> HSELLVN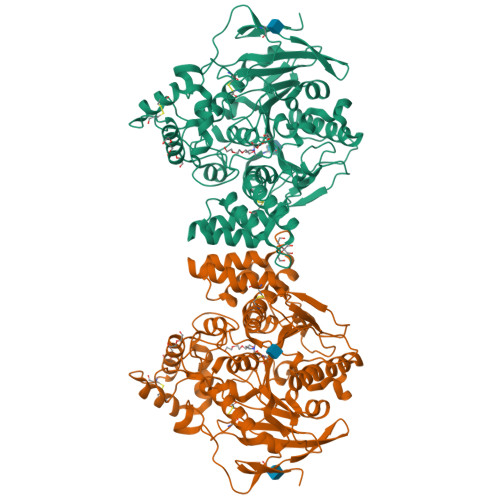TKSGKVMGTRVPVLSSHISAFLGIPFAEPPVGNMRFRRPEPKKPWSGVWNASTYPNNCQQYVDEQFPGFSGSEMWNPNREMSEDCLYLNIWVPSPRPKSTTVMVWIYGGGFYSGSSTLDVYNGKYLAYTEEVVLVSLSYRVGAFGFLALHGSQEAPGNVGLLDQRMALQWVHDNIQFFGGDPKTVTIFGESAGGASVGMHILSPGSRDLFRRAILQSGSPNCPWASVSVAEGRRRAVELGRNLNCNLNSDEELIHCLREKKPQELIDVEWNVLPFDSIFRFSFVPVIDGEFFPTSLESMLNSGNFKKTQILLGVNKDEGSFFLLYGAPGFSKDSESKISREDFMSGVKLSVPHANDLGLDAVTLQYTDWMDDNNGIKNRDGLDDIVGDHNVICPLMHFVNKYTKFGNGTYLYFFNHRASNLVWPEWMGVIHGYEIEFVFGLPLVKELNYTAEEEALSRRIMHYWATFAKTGNPNEPHSQESKWPLFTTKEQKFIDLNTEPMKVHQRLRVQMCVFWNQFLPKLLNAT> DLQLLHQKVEEQAAKYKHRVPKKCCYDGARENKY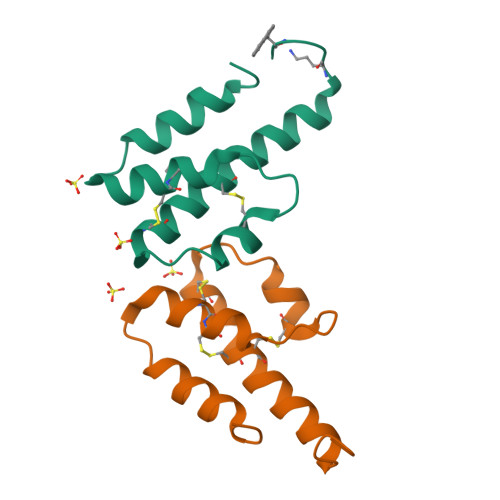ETCEQRVARVTIGPHCIRAFNECCTIADKIRKNISHKFAPAAR;> DLQLLHQKVEEQAAKYKHRVPKKCCYDGARENKYETCEQRVARVTIGPHCIRAFNECCTIADKIRKESHHKGMLLGR>[2x]MGSSHHHHHHSSGLVPRGSHMPSASASRKSQEKPREIMDAAEDYAKERYGISSMIQSQEKPDRVLVRVRDLTIQKADEVVWVRARVHTSRAKGKQCFLVLRQQQFNVQALVAVGDHASKQMVKFAANINKESIVDVEGVVRKVNQKIGSCTQQDVELHVQKIYVISLAEPRLPLQLDDAVRPEAEGEEEGRATVNQDTRLDNRVIDLRTSTSQAVFRLQSGICHLFRETLINKGFVEIQTPKIISAASEGGANVFTVSYFKNNAYLAQSPQLYKQMCICADFEKVFSIGPVFRAEDSNTHRHLTEFVGLDIEMAFNYHYHEVMEEIADTMVQIFKGLQERFQTEIQTVNKQFPCEPFKFLEPTLRLEYCEALAMLREAGVEMGDEDDLSTPNEKLLGHLVKEKYDTDFYILDKYPLAVRPFYTMPDPRNPKQSNSYDMFMRGEEILSGAQRIHDPQLLTERALHHGIDLEKIKAYIDSFRFGAPPHAGGGIGLERVTMLFLGLHNVRQTSMFPRDPKRLTP

Aminoacyl-tRNA synthetases (AARSs) catalyze the attachment of respective amino acid substrate to its cognate tRNA through a two-step reaction. In human, there are cytosolic and mitochondrial aspartyl-tRNA synthetases (DRS and DRS2), which share only 22.9% sequence identity. In the case of DRS, it is one of the components that forms the multi-tRNA synthetase complex (MSC) in higher eukaryotes. In the MSC, DRS is known to interact with the AARS-interacting multifunctional protein 2 (aminoacyl-tRNA synthetase-interacting multifunctional protein AIMP2/p38)8,9 and the lysyl-tRNA synthetase (KRS).

In this study, we present the crystal structure of human cytosolic DRS at 2.25 Å. We show that DRS forms a homodimer with the N-terminal extension, anticodon-binding domain, hinge region, and catalytic domain. DRS contains a homodimer in the asymmetric unit and the dimer interface area is 3750.5 Å2 which comprises 16.6% of the monomeric surface area calculated from Protein Interfaces, Surfaces, and Assemblies service. Our crystal structure includes all the Class II AARS domains: anticodon-binding domain, hinge region, and catalytic domain. In addition, the N-terminal extension, which is a distinct domain in mammalian DRS, could be partially modeled including the C-terminal three residues of the characteristic helix motif [Fig. 1(A)]. The anticodon-binding domain of DRS (residues, 57–146) adopts the oligonucleotide binding-fold (OB-fold) that is composed of a five-stranded antiparallel β-sheet connected by helices and loops (β1–β5) to form a closed β-barrel. The catalytic domain (residues, 189–497) contains 13 α-helices (αH–αT) and 8 β-strands (β6–β13) which constitute all the three conventional Class II AARS motifs: Motifs 1, 2, and 3.2 The hinge region (residues, 156–188) plays an essential role in the connection of the anticodon-binding domain and the catalytic domain. In the middle of the hinge region, residues 163–172 could not be modeled owing to the lack of the electron density and the disordered residues are considered as a part of binding region to the ribose-phosphate backbone in the D-stem of tRNAAsp, compared with the known S. cerevisiae DRS–tRNAAsp complex structure. In addition, residues 224–247 in the flipping loop and residues 273–282 in the Motif 2 could not be observed in our crystal structure [Fig. 1(B)]. Thus, we suggest that the phosphorylation of Ser146 could initiate a conformation change of the DRS dimer and trigger an unpredicted function of DRS by releasing it from the MSC.>[2x]GANDHVPS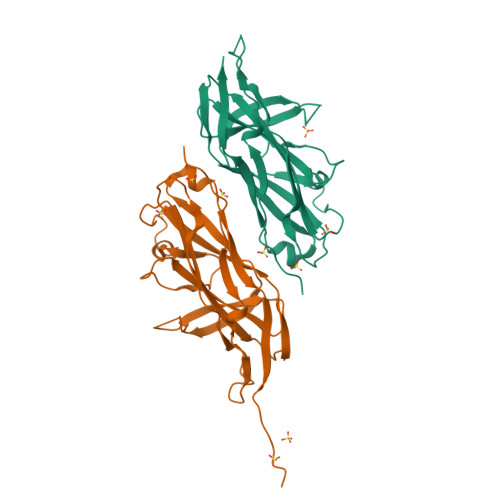PITINTSTLPVVVIGPADAHTYPRVIGELTGTSNQYIFNGGSLIALMRGKFTPTLPKIGKITYNFRQGNNTQSSDFDIFDTGVPGLGIIIGMAGYWPATPLVPINSSSIYIDPVAANTNPNAYNGATGSFGARLYVAFVATGRLPNGYVTIPTKQLGHILLESNRASLNNKRLTAPVMLNGGRIQVQSQAHHHHHH>MGAEEEDTAILYPFTISGNDRNGNFTINFKGTPNSTNNGCIGYSYNGDWEKIEWEGSCDGNGN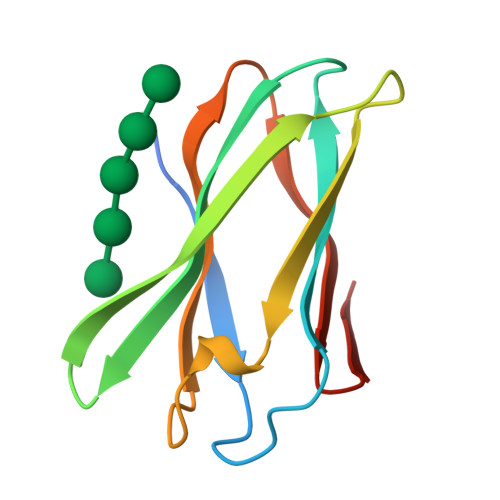LVVEVPMSKIPAGVTSGEIQIWWHSGDLKMTDYKALEHHHHHH[2x]>GAMVSQPIKLLVGLANPGPEYAKTRHNAGAWVVEELARIHNVTLKNEPKFFGLTGRLLINSQELRVLIPTTFMNLSGKAIAALANFYQIKPEEIMVAHDELDLPPGVAKFKQGGGHGGHNGLKDTISKLGNNKEFYRLRLGIGHPGHKDKVAGYVLGKAPAKEQECLDAAVDESVRCLEI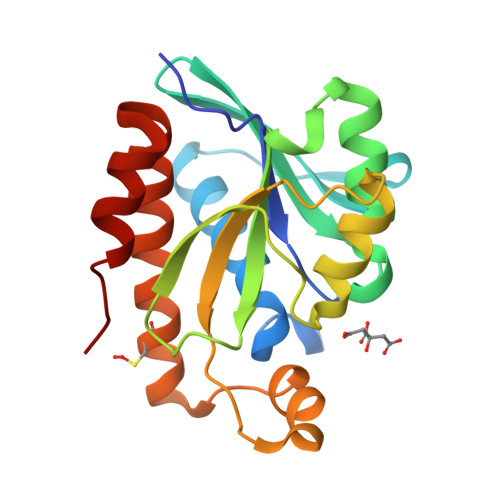LMKDGLTKAQNRLHTFKAE[2x]> NAIMDLQTRNTRGLSTLVVRDIGELMMAGDMAVIERYVADVRGKGAVLDLRIYDAAGRPAGKKQDAPDGEVQAALTSGATAEKRHKVDGRHVLSFIVP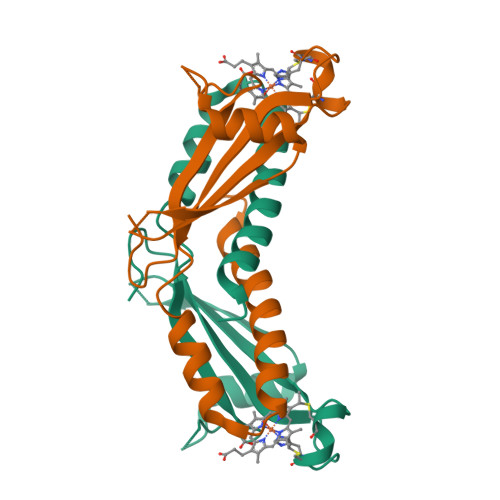LANEVRCQSCHEQGARFNGAMLLTTSLEEGYAGARN N-acetyl-beta-D-glucopyranosylamine | C8 H15 N O6 | 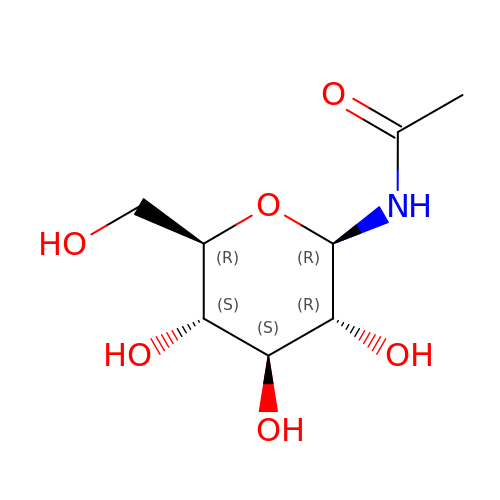IBONACLSSOLHFU-JAJWTYFOSA-N Here, we show that Pseudomonas aeruginosa OprC is an outer membrane, TonB-dependent transporter that is conserved in many Proteobacteria and which mediates acquisition of both reduced and oxidised ionic copper via an unprecedented CxxxM-HxM metal binding site. As indicated by the successful structure solution, OprC contains a single bound copper and shows the typical fold of a TBDT, with a large 22-stranded β-barrel occluded by an N-terminal approximately 15 kDa plug domain that, like in other TBDTs, completely occludes the lumen of the barrel. The copper binding site comprises residues Cys143 and Met147 in the plug domain and His323 and Met325 in the barrel wall. The CxxxM-HxM configuration, which coordinates the copper in a tetrahedral manner, is highly unusual and has, to our knowledge, not been observed before in copper homeostasis proteins.

Interestingly, the active site His117 in azurin renders the copper atom solvent inaccessible, reminiscent to the likely role of Met147 in OprC. The superficial similarity of the OprC binding site to that of (pseudo)azurin prompted us to generate the M147H and M325H OprC mutants in an attempt to convert OprC into a unique, blue copper transport protein. However, in the presence of added Cu(II), both mutants remain colourless, and comparison of the crystal structures with those of pseudoazurin and plastocyanin show small but most likely important differences in the geometries of the active sites.

>MEKRMSTQQRAAGNACPTAAFSFDPARLAQRRRWAGAFAALCGLALSPSALLAEEHSQHQDHAVELAPSVVTGVAQSSPLTIVTNPKEPRQPVPASDGADYLKTIPGFAVIRNGGSNGDPVLRGMFGSRLNILTNGGMMLGACPNRHDAPTSYISPETYDKLTVIKGPQTVLWGPGASAGTILFEREPERFGELGSRVNASLLAGSNGRFDKVLDAAAGNRLGYLRFTGNHAQSDDYEDGAGNTVPSRWKKWNGDVAVGWTPDEDTLIELTAGKGDGEARYAGRGMDGSQFKRESLGLRFVKSNVSDVLEKVEAQVYYNYADHIMDNFRLRTPDPSSMMPMPMASQVDRRTLGGRLAATWRWDDFKLVTGVDAMRNEHRARGSKYDMMTDYYTDADQFPWSKDAVFHNYGAFGELTWFAAERDRLIGGLRLDRASVKDYRQTLKSGHMGHAMANPTANDTRADTLPSGFVRYEHDLADSPTTLYAGLGHAERFPDYWELFSPKRGPNGSVNAFDKIKPEKTTQLDFGLQYNGDKLQAWASGYVGVVQDFILFSYREGMMGSSTQATNVDARIMGGELGASYQLTGNWKTDASLAYAWGKNSSDDRALPQIPPLEARFGLTYEEGDWSAGSLWRVVAPQNRIARDQGNVVGKDFDKSAGFGVFSLNGAYRVTRNVKLSAGVDNLFDKDYTEHLNKAGDAGFGFSANETVPEPGRTFWTKVDFSF[2x]N-(4-AMINO-5-CYANO-6-ETHOXYPYRIDIN-2-YL)-2-(4-BROMO-2,5-DIMETHOXYPHENYL)ACETAMIDE 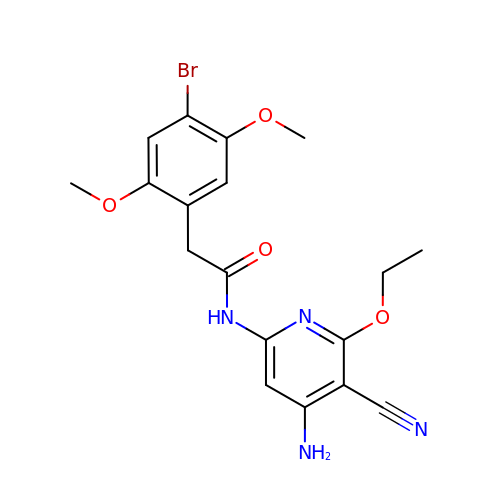| C18 H19 Br N4 O4 | GKODDLYLEKSDJL-UHFFFAOYSA-N>[4x]MLCEIECRALSTAHTRLIHDFEPRDALTYLEGKNIFTEDHSELISKMSTRLERIANFLRIYRRQASELGPLIDFFNYNNQSHLADFLEDYIDFAINEPDLLRPVVIAPQFSRQMLDRKLLLGNVPKQMTCYIREYHVDRVIKKLDEMCDLDSFFLFLHGRAGSGKSVIASQALSKSDQLIGINYDSIVWLKDSGTAPKSTFDLFTDILLMLKSEDDLLNFPSVEHVTSVVLKRMICNALIDRPNTLFVFDDVVQEETIRWAQELRLRCLVTTRDVEISNAASQTCEFIEVTSLEIDEC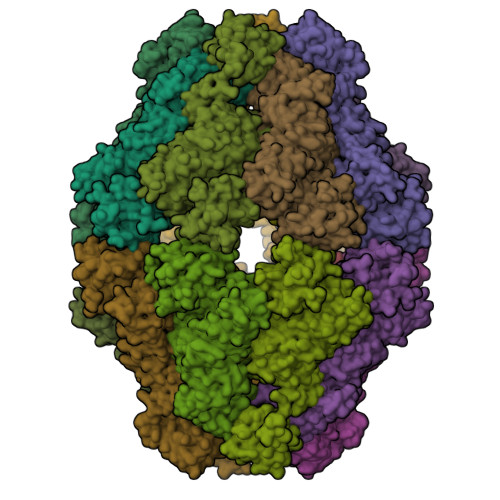YDFLEAYGMPMPVGEKEEDVLNKTIELSSGNPATLMMFFKSCEPKTFEKMAQLNNKLESRGLVGVECITPYSYKSLAMALQRCVEVLSDEDRSALAFAVVMPPGVDIPVKLWSCVIPVDICSNEEEQLDDEVADRLKRLSKRGALLSGKRMPVLTFKIDHIIHMFLKHVVDAQTIANGISILEQRLLEIGNNNVSVPERHIPSHFQKFRRSSASEMYPKTTEETVIRPEDFPKFMQLHQKFYDSLKNFACC;>[4x]PMFNFLGC>MADSTFLAPELSDTESMGEETVRFQELLLKASKELQQAQTARPDSTQIQPKPGFCVKTNSSEGKVFINICHSPSIPPPADVTEDELLQMLEEDQAGFRIPMSLGEPHAELDAKGQGCTAYDVAVNSNFYLRMQNSDFLRELVVTIAREGLEDKYGLQLNPEWRMLKYRSFLGSISQQNIRSQQRPRIQELGTLDASGSLG[2x];>[2x]ELDSDDEFS

The R2TP complex is found in organisms from yeast to humans, and consists of the AAA+ ATPases Rvb1 and Rvb2 (human: RUVBL1 and RUVBL2), a TPR-containing protein, Tah1 (human: Spagh or RPAP3), and Pih1 (also known as NOP17 and Pih1D1, but referred to as Pih1 henceforth; Kakihara and Houry, 2012; Te et al., 2007). Pih1 is the multipoint scaffold of the R2TP complex, coupling the Rvb1-Rvb2 hetero-dodecamer, the Hsp90 chaperone machinery (via Tah1 in yeast or Spagh/RPAP3 in metazoa), and the TTT (Tel2-Tti1-Tti2) complex implicated in activation and stabilization of PIKKs (Hurov et al., 2010; Kakihara and Houry, 2012). The biological roles ascribed to the R2TP complex are directly associated with its ability to interact with the Hsp90 chaperone system and function as an Hsp90 cochaperone (Boulon et al., 2010; Izumi et al., 2012; Takai et al., 2010). Here we present crystal structures of Hsp90-Tah1-Pih1, Hsp90-Spagh/RPAP3, and Pih1-Tel2 complexes that together define key structural links within the R2TP core in yeast and in animals and reveal how R2TP connects the Hsp90 chaperone system to the TTT complex involved in PIKK activation.

Interaction with Tel2 involves the N-terminal segment of Pih1 (Horejsí et al., 2010), which contains a conserved region of unknown structure (henceforth, PIH domain). We determined the crystal structure of the mouse PIH domain1–200 with single-wavelength anomalous dispersion phasing of Tel2-peptide cocrystals (see below) grown with SeMet protein (see Experimental Procedures) and used this to phase the mPih47–179 apo and SELDpSDDEF peptide-bound structures, which were refined to 2.1 and 3.3 Å, respectively. We next obtained crystals of a complex of the PIH domain and the Ser 488-Ser 492-bis-phosphorylated Tel2 peptide. The PIH domain consists of a twisted five-stranded β sheet with one face traversed by a helix-turn-helix segment connecting strands 4 and 5, and the other face traversed by a coil segment extending from the end of β strand 5. The interaction of the PIH domain and the Tel2 phosphopeptide is highly unusual when compared with other known phosphopeptide binding domains. The phosphoserine phosphate group and the side chain carboxyls of the flanking aspartic acid residues on the Tel2 peptide cooperate in an interconnecting network of polar interactions with lysine residues 57 and 64 in the PIH domain. An additional interaction with the PIH domain main chain is provided by the aspartic acid side chain +2 relative to the phosphoserine. An additional source of specificity may be contributed by the hydrophobic interaction of Tel2-Phe 496, positioned +4 relative to the phosphoserine. The PIH domain itself and its mode of binding to the Tel2 phosphopeptide are distinct from previously reported phosphoserine/phosphothreonine-binding domains such as BRCT or FHA domains (Ali et al., 2009; Kilkenny et al., 2008; Qu et al., 2013).>MSTNKVNKERTFLAVKPDGVARGLVGEIIARYEKKGFVLVGLKQLVPTKDLAESHYAEHKERPWFGGLVSFITSGPVVAMVFEGKGVVASARLMIGVTNPLASAPGSIRGDFGVDVGRSIIGGSDSVESANREIALWFKPEELLTEVKPNPNLYE[2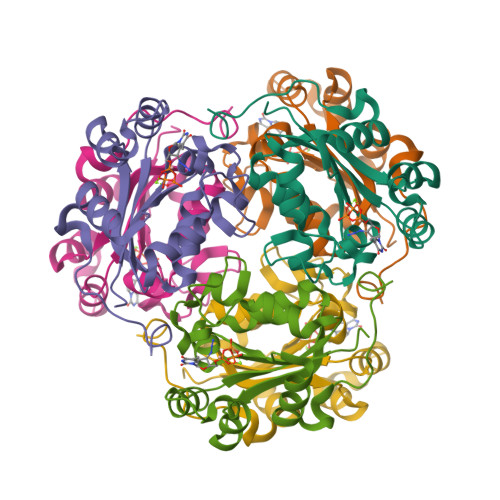x]>[6x]MGSMEAERVRVFHKQAFEYISIALRIDEDEKAGQKEQAVEWYKKGIEELEKGIAVIVTGQGEQCERARRLQAKMM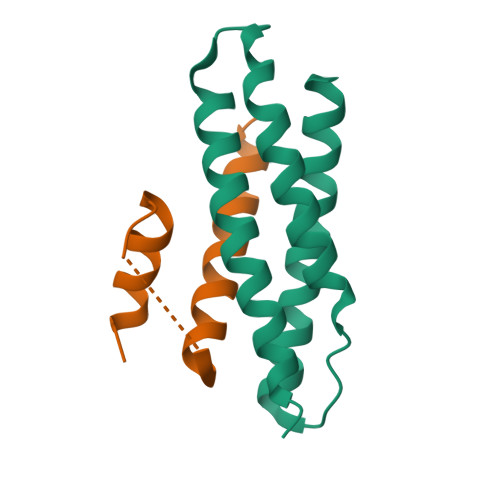TNLVMAKDRLQLLE;>QVDMLLQEMADEAGLDLNMELPQGQTGSVGTSVASAEQDELSQRLARLRD[6x]> MKDLLKFLKAQTKTEEFDAIKIALASPDMIRSWSFGEVKKPETINYRTFKPERDGLFCARIFGPVKDYECLCGKYKRLKHRGVICEKCGVEVTQTKVRRERMGHIELASPTAHIWFLKSLPSRIGLLLDMPLRDIERVLYFESYVVIEGGMTNLERQQILTEEQYLDALEEFGDEFDAKMGAEAIQALLKSMDLEQECEQLREELNETNSETKRKKLTKRIKLLEAFVQSGNKPEWMILTVLPVLPPDLRPLVPLDGGRFATSDLNDLYRRVINRNNRLKRLLDLAAPDIIVRNEKRMLQEAVDALLDNGRRGRAITGSNKRPLKSLADMIKGKQGRFRQNLLGKRVDYSGRSVITVGPYLRLHQCGLPKKMALELFKPFIYGKLELRGLATTIKAAKKMVEREEAVVWDILDEVIREHPVLLNRAPTLHRLGIQAFEPVLIEGKAIQLHPLVCAAYNADFDGDQMAVHVPLTLEAQLEARALMMSTNNILSPANGEPIIVPSQDVVLGLYYMTRDCVNAKGEGMVLTGPKEAERLYRSGLASLHARVKVRITEYEKDANG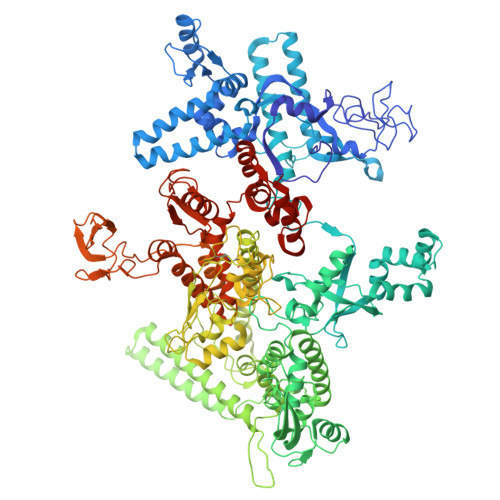ELVAKTSLKDTTVGRAILWMIVPKGLPYSIVNQALGKKAISKMLNTCYRILGLKPTVIFADQIMYTGFAYAARSGASVGIDDMVIPEKKHEIISEAEAEVAEIQEQFQSGLVTAGERYNKVIDIWAAANDRVSKAMMDNLQTETVINRDGQEEKQVSFNSIYMMADSGARGSAAQIRQLAGMRGLMAKPDGSIIETPITANFREGLNVLQYFISTHGARKGLADTALKTANSGYLTRRLVDVAQDLVVTEDDCGTHEGIMMTPVIEGGDVKEPLRDRVLGRVTAEDVLKPGTADILVPRNTLLHEQWCDLLEENSVDAVKVRSVVSCDTDFGVCAHCYGRDLARGHIINKGEAIGVIAAQSIGEPGTQLTMRTFHIGGAASRAAAESSIQVKNKGSIKLSNVKSVVNSSGKLVITSRNTELKLIDEFGRTKESYKVPYGAVLAKGDGEQVAGGETVANWDPHTMPVITEVSGFVRFTDMIDGQTITRQTDELTGLSSLVVLDSAERTAGGKDLRPALKIVDAQGNDVLIPGTDMPAQYFLPGKAIVQLEDGVQISSGDTLARIPQESGGTKDITGGLPRVADLFEARRPKEPAILAEISGIVSFGKETKGKRRLVITPVDGSDPYEEMIPKWRQLNVFEGERVERGDVISDGPEAPHDILRLRGVHAVTRYIVNEVQDVYRLQGVKINDKHIEVIVRQMLRKATIVNAGSSDFLEGEQVEYSRVKIANRELEANGKVGATYSRDLLGITKASLATESFISAASFQETTRVLTEAAVAGKRDELRGLKENVIVGRLIPAGTGYAYHQDRMRRRAAGEAPAAPQVTAEDASASLAELLNAGLGGSDNE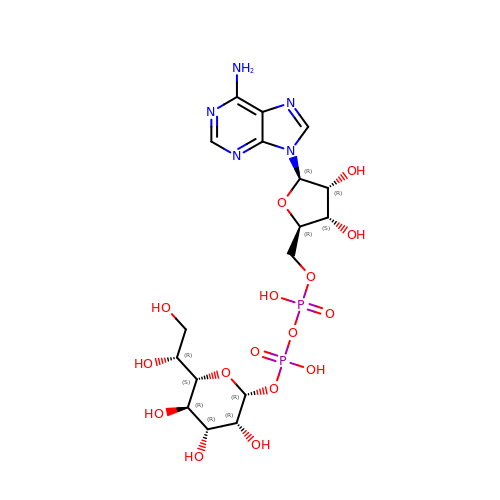[(2R,3S,4R,5R)-5-(6-amino-9H-purin-9-yl)-3,4-dihydroxytetrahydrofuran-2-yl]methyl (2R,3R,4R,5R,6S)-6-[(1R)-1,2-dihydroxyethyl]-3,4,5-trihydroxytetrahydro-2H-pyran-2-yl dihydrogen diphosphate | C17 H27 N5 O16 P2 | KMSFWBYFWSKGGR-GZNZTODLSA-N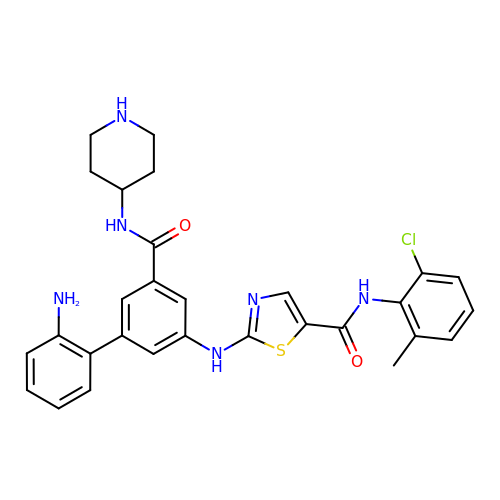2-[[3-(2-aminophenyl)-5-(piperidin-4-ylcarbamoyl)phenyl]amino]-~{N}-(2-chloranyl-6-methyl-phenyl)-1,3-thiazole-5-carboxamide | C29 H29 Cl N6 O2 S | IPDDCJRBTYYNRD-UHFFFAOYSA-N>GAMTIGRAKVYATLSKIFYHLFYDEAIPKDCREIIEKFGEIDFNLRSVLVRELRGSVLIKDMPQSLAEVYESVMKDFYERYGFQASELHADHIAVELAFMSKLVEREISLAQQMKEEELYKIRAAQHRFIKAHLQPLVKNLPSAPLLNFVRDFVREDAKYLYSSLVGEKNEG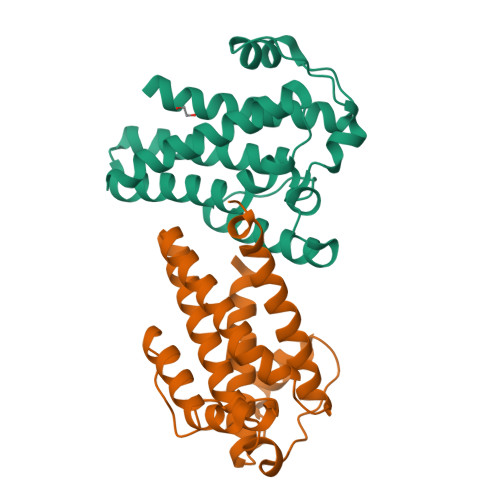ADNN[2x]(2~{S},3~{R})-2-(hydroxymethyl)piperidin-3-ol 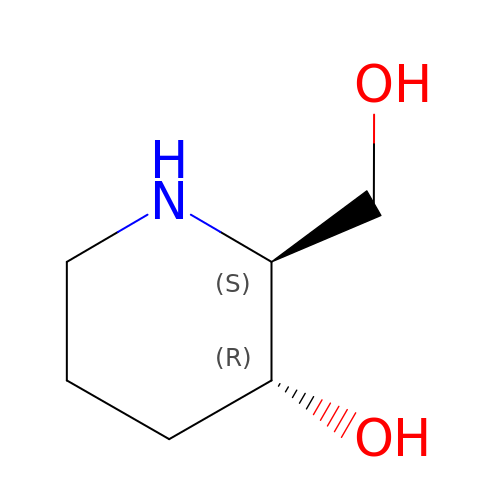| C6 H13 N O2 | WRLZCUCTSFUOQY-NTSWFWBYSA-N> MFSLPTLTSDITVEVNSSATKTPFVRRPVEPVGKFFLQHAQRTLRNHTWSEFERIEAEKNVKTVDESNVDPDELLFDTELADEDLLTHDARDWKTADLYAAMGLSKLRFRATESQIIKAHRKQVVKYHPDKQSAAGGSLDQDGFFKIIQKAFETLTDSNKRAQYDSCDFVADVPPPKKGTDYDFYEAWGPVFEAEARFSKKTPIPSLGNKDSSKKEVEQFYAFWHRFDSWRTFEFLDEDVPDDSSNRDHKRYIERKNKAARDKKKTADNARLVKLVERAVSEDPRIKMFKEEEKKEKERRKWEREAGARAEAEAKAKAEAEAKAKAESEAKANASAKADKKKAKEAAKAAKKKNKRAIRNSAKEADYFGDADKATTIDEQVGLIVDSLNDEELVSTADKIKANAAGAKEVLKESAKTIVDSGKLPSSLLSYFV;> MSSPVIGITFGNTSSSIAYINPKNDVDVIANPDGERAIPSALSYVGEDEYHGGQALQQLIRNPKNTIINFRDFIGLPFDKCDVSKCANGAPAVEVDGKVGFVISRGEGKEEKLTVDEVVSRHLNRLKLAAEDYIGSAVKEAVLTVPTNFSEEQKTALKASAAKIGLQIVQFINEPSAA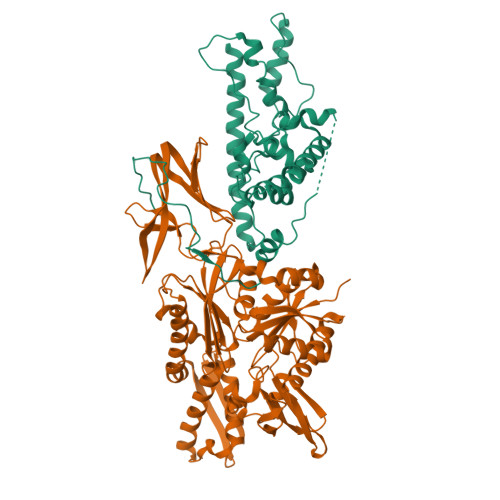LLAHAEQFPFEKDVNVVVADFGGIRSDAAVIAVRNGIFTILATAHDLSLGGDNLDTELVEYFASEFQKKYQANPRKNARSLAKLKANSSITKKTLSNATSATISIDSLADGFDYHASINRMRYELVANKVFAQFSSFVDSVIAKAELDPLDIDAVLLTGGVSFTPKLTTNLEYTLPESVEILGPQNKNASNNPNELAASGAALQARLISDYDADELAEALQPVIVNTPHLKKPIGLIGAKGEFHPVLLAETSFPVQKKLTLKQAKGDFLIGVYEGDHHIEEKTLEPIPKEENAEEDDESEWSDDEPEVVREKLYTLGTKLMELGIKNANGVEIIFNINKDGALRVTARDLKTGNAVKGEL> MKWSEYANLAQQSLEKFYLADTKEQFLNNFYPTENPEEDNKVFNYWWLAHLVEVRLDAYLRTKKQADLEVAEKTYLHNKNRNGGTLIHDFYDDMLWNALAAYRLYKATGKSIYLEDAQLVWQDLVDTGWNDIMGGGFAWRRPQMYYKNTPVNAPFIILSCWLYNELNETKYLEWAMKTYEWQTKVLVREDGFVEDGINRLEDGTIDYEWKFTYNQGVYIGANLELYRITKEAIYLDTANKTAAISLKELTEDGIFKDEGNGGDEGLFKGIFYRYFTDLIEETANKTYRDFVLNSCQILVENAKLDGY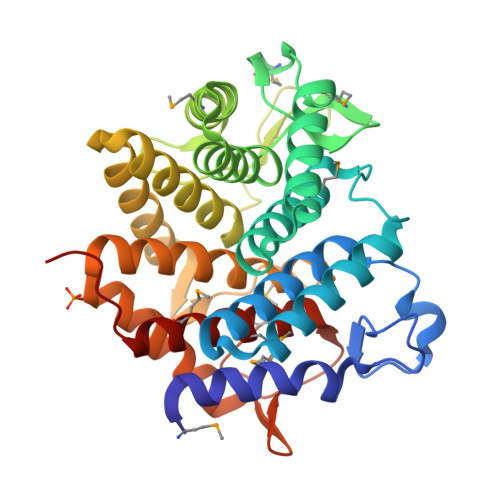LLMGMNWKEKPSGKIPYSAELSGMIALEMAAKLELEHHHHHH1H-INDOL-3-YLACETIC ACID | C10 H9 N O2 | 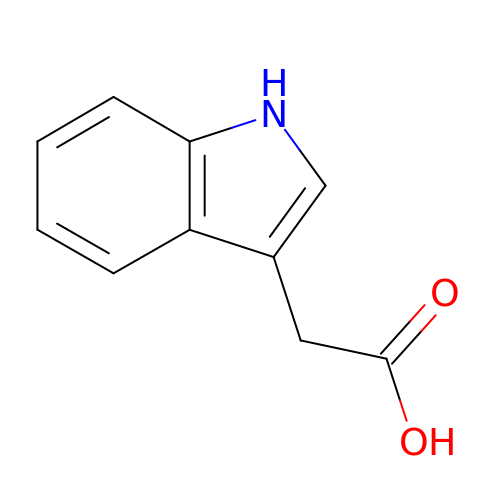SEOVTRFCIGRIMH-UHFFFAOYSA-N The conserved shelterin complex caps chromosome ends to protect telomeres and regulate telomere replication. In fission yeast Schizosaccharomyces pombe, shelterin consists of telomeric single- and double-stranded DNA-binding modules Pot1-Tpz1 and Taz1-Rap1 connected by Poz1, and a specific component Ccq1. Here, we report the crystal structures of Pot1DBD-single-stranded-DNA, Pot1372-555-Tpz1185-212 and Tpz1425-470-Ccq1123-439 complexes and propose an integrated model depicting the assembly mechanism of the shelterin complex at telomeres. Overall, our findings provide valuable structural information regarding interactions within fission yeast shelterin complex at 3’ ss telomeric overhang.

After an extensive screening of deletion mutations, we identified a construct of Ccq1123-439 with a deletion of residues 199–215 (Ccq1123-439 Δ199–215), which could form a stable binary complex with Tpz1425-470 and produce high-quality crystals for structural studies. We determined the Tpz1CBM-Ccq1TAD complex structure by the SAD method at a resolution of 2.4 Å. The Tpz1CBM-Ccq1TAD complex structure reveals a 2:2 stoichiometry and buries a total of ~2,100 Å2 surface area in the complex. The Tpz1CBM-Ccq1TAD complex exhibits a butterfly-shaped architecture with two Ccq1TAD molecules as the ‘wings’ and Tpz1CBM as the ‘antenna’. The two Tpz1CBM polypeptides adopt symmetric conformations and each Tpz1CBM contains an N-terminal loop and a C-terminal helix, which respectively interact with the two Ccq1TBM molecules in the heterotetamer complex. In the center of the Tpz1CBM-Ccq1TAD complex, the two Ccq1TAD molecules mediate a dimeric contact in a head-to-head fashion, burying ~500 Å2 surface area between the two monomers. In the Tpz1CBM-Ccq1TAD complex, the N-terminal loop of Tpz1CBM adopts an extended conformation, meandering in a shallow, acidic groove formed by helices α2 and α10 as well as the C-terminal end of one Ccq1TAD molecule, primarily stabilized by a panel of electrostatic and hydrogen-bonding interactions. The Tpz1CBM polypeptide makes a sharp turn at Asp438 and Tyr439 so that the C-terminal helix makes direct contacts with the other Ccq1TAD monomer in the complex. The hydrophobic portion of the amphipathic helix of Tpz1CBM fits into a long groove formed by helices α1, α3 and α4 of Ccq1TAD through extensive hydrophobic contacts. Collectively, we conclude that hydrophobic contacts at the interface are the major driving force underlying the Ccq1-Tpz1 interaction.

>[2x]ITKSSKSSFSVLDIGLPMSALQRKMMHRLVQYFAFCIDHFCTGPSDSRIQEKIRLFIQSAHNIAKHPSLYDTEVRNPSAAESTNSHVSLDASNFSSYAENSSKFLFLQELFKNLSPSYSKTFFLFISNQFLANTLTQWLKSQNIDAELWAEEDAKTSQHPAIWICVSKKAPSASHFLQSCPDLSATIFYDIEAYMSVTSSLPSIQSLVLRLIHLGSIEHAIKCFQSSYNASFLVNIVGVVATLSSSSEENSEASNLSTLFEKSGNFEEILGSESHSSITEKTRDIAKNVATWLKNGENFSSWPLPPLMDLASLSVAE;>QIELEYKRKPIPDYDFMKGLETTLQELYVEHQSKKRRLELFQLTN[2x]>[2x]MNIVVLISGNGSNLQAIIDACKTNKIKGTVRAVFSNKADAFGLERARQAGIATHTLIASAFDSREAYDR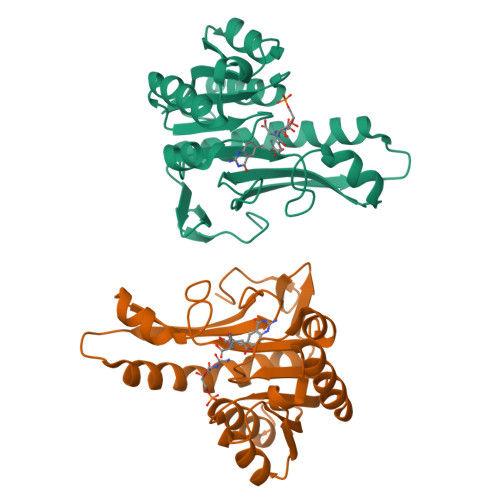ELIHEIDMYAPDVVVLAGFMRILSPAFVSHYAGRLLNIHPSLLPKYPGLHTHRQALENGDEEHGTSVHFVTDELDGGPVILQAKVPVFAGDSEDDITARVQTQEHAIYPLVISWFADGRLKMHENAAWLDGQRLPPQGYA>MAGRLREMRCELSFLKNADGSACFSQGATCIWASCSGPGDVHASKASDEAMTLDISYRANCGDNKFNVLNNIIHSTLSNAINLELFPHTTISVTVHGIQDDGSMGAVAINGACFALLDNGMPFETVFCGVLIVRVKDELIIDPTAKQEAASTGRVLFSVCKGSDGHPEVCAMDAIGHWDFIQLEAAWSLAQPS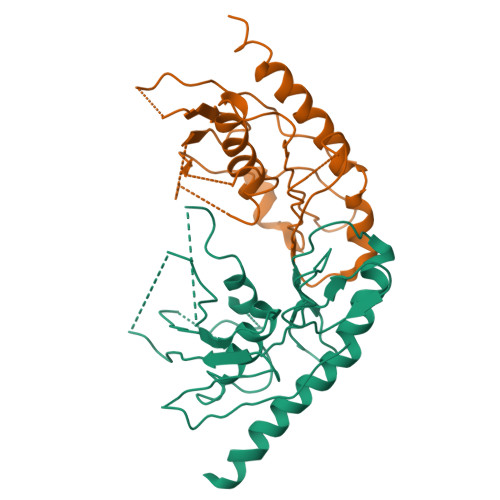ASAIFDFYKTVMKRKLSVDEQLEHHHHHH[2x]> MDGSGEQPRGGGPTSSEQIMKTGALLLQGFIQDRAGRMGGEAPELALDPVPQDASTKKLSESLKRIGDELDS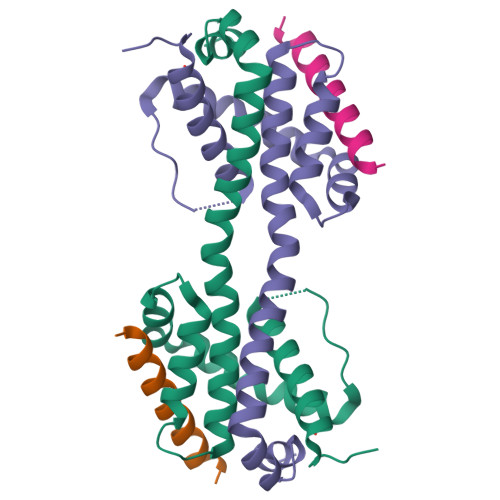NMELQRMIAAVDTDSPREVFFRVAADMFSDGNFNWGRVVALFYFASKLVLKALSTKVPELIRTIMGWTLDFLRERLLGWIQDQGGWDGLLSYFGSS;> DMRPEIWIAQELRRIGDEFNAYYARR ADENOSINE-5'-MONOPHOSPHATE 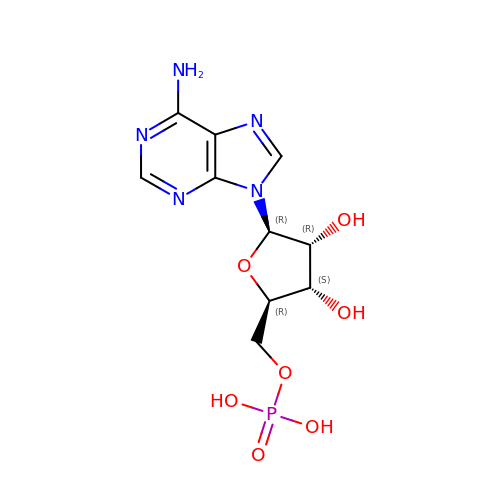| C10 H14 N5 O7 P | UDMBCSSLTHHNCD-KQYNXXCUSA-N> MSAKL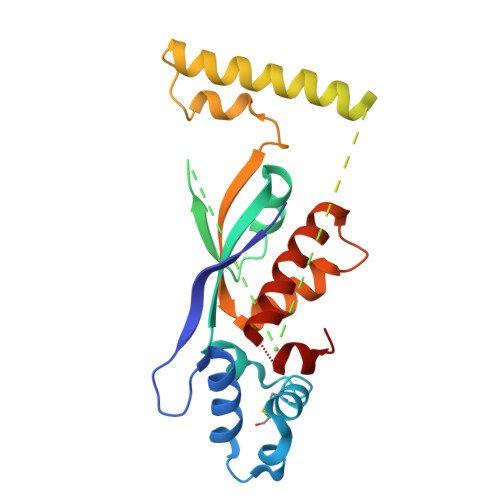ISVTKPVVEGVNTAEELIAYAARVSNPENQINNKTASGLLKYCIRHKHWSIFETAFMTLELKTSRGIAAQVIRHRSFHFQEFSQRYASVMETPPPHQARFQDHKNRQNSLDTVPEDDQTWWATEQEKLYAQSMELYNKALEKGIAKECARFILPLSTPTTIYMSGTIRDWIHYIELRTSNGTQREHIDLANACKEIFIKEFPSIAKALDWVH> MVSTRETVNELLRRIAAGDPGRIAELYAEEVSWKLSWPAGDHMGVVPWIQ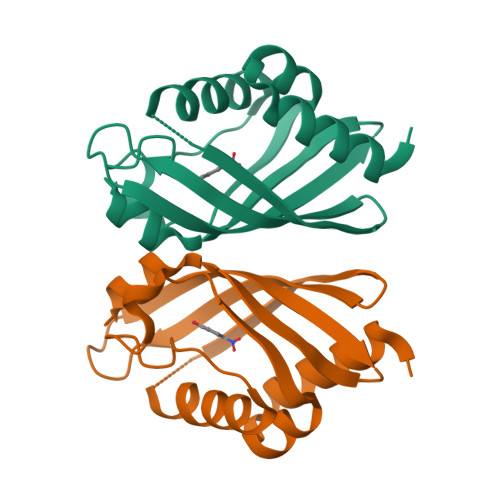QRSTRAGVEEHFRLIADHHVAKQSSAEVFSVLVDGADAVVLGELRNTAGPTGRSYEAPFALHLTVENGLVTRHHVYEDSLAVFRAFAENAGEPVRSRAS>MGSGLKAGDSFPSDVVFSYIPWSEDKGEITACGIPINYNASKEWADKKVILFALPGAFTPVCSARHVPEYIEKLPEIRAKGVDVVAVLAYNDAYVMSAWGKANQVTGDDILFLSDPDARFSKSIGWADEEGRTKRYALVIDHGKITYAALEPAKNHLEFSSAETVLKHLHHHHHH[2x]

The intracellular Asp f3 is an abundant protein in A. fumigatus. It contains 168 amino acid residues and BLAST searches reveal considerable sequence homology to the thioredoxin superfamily, the peroxiredoxin (Prx) family, and the PRX5-like subfamily. We experimentally confirm the predicted peroxiredoxin activity of Asp f3 and demonstrate the functional contribution of its cysteine residues for catalytic activity. Finally, we provide evidence for the critical role of Asp f3 in fungal virulence, wherein it protects A. fumigatus against oxidative stress in vitro, and in vivo, in a murine model of invasive pulmonary aspergillosis.

Aspf3 wild type (WT) and its C31S/C61S variant crystallized as a homodimer and showed a typical thioredoxin-like fold. The WT protein was captured in its oxidized state, with two intermolecular disulfide bonds across the dimerization interface between C31 and C61 of the individual protomers. In the WT structure, both C31 and C61 reside in flexible loop regions (large B-factors and lack of well-defined electron density for one of the chains). The crystal structure of Asp f3 revealed its homodimeric configuration that includes two intermolecular disulfide bonds. The dimer interface comprises an area of ~710 Å2 and ~730 Å2 for WT and C31S/C61S variant, respectively. Salt bridges between R131 and D91 from the two protomers and additional hydrogen bonds between main chain atoms (T29-V60, A30-V60, A30-C61), as well as residues involved in hydrophobic interactions (I28, A30, F57, P59, V60, V94, Y93, A97) contribute to the extensive interface interactions. The WT, as well as C31S/C61S variant, exhibited close similarity to oxidized and reduced forms of Ahp1, respectively. The residue at the active site (C61) is the peroxidatic cysteine (CP) that initiates the peroxide reduction by nucleophilic attack, when present in its thiolate form. The second Cys residue (C31) is therefore designated as the resolving cysteine (CR) that participates in catalysis in later reaction step. Disulfide reductases such as a thioredoxin or glutaredoxin return oxidized Asp f3 to its activated, reduced state.2-ethyl-~{N}-[(1~{S})-4-(2-fluoranylethanimidoylamino)-1-(4-methoxy-1-methyl-benzimidazol-2-yl)butyl]-3-oxidanylidene-1~{H}-isoindole-4-carboxamide | C26 H31 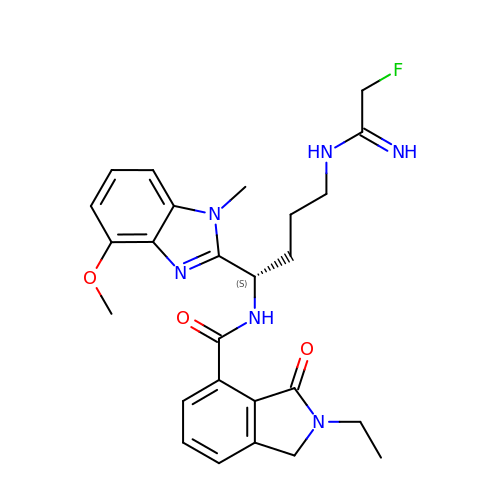F N6 O3 | OVAMJGKJUQRQOY-SFHVURJKSA-N> GSHMLEPELKVGIVGNLASGKSALVHRYLTGTYVQEESPEGGRFKKEIVVDGQSYLLLIRDEGGPPEAQFAMWVDAVIFVFSLEDEISFQTVYHYYSRMANYRNTSEIPLVLVGTQDAISSANPRVIDDARARKLSNDLKRCTYYETCATYGLNVERVFQDVAQKIVA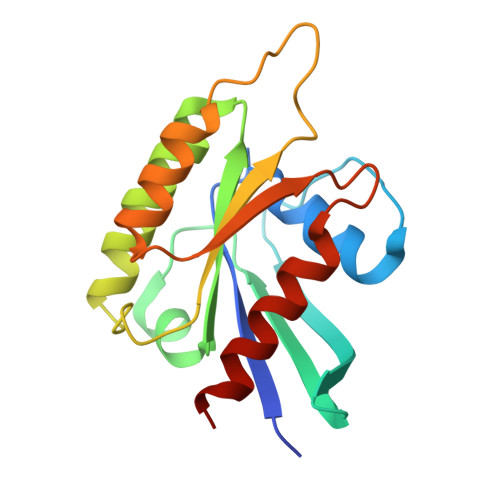TRKK> MEKIKVAIADDNKELVKTLESYLADHPQIEVITTAPNGKVILS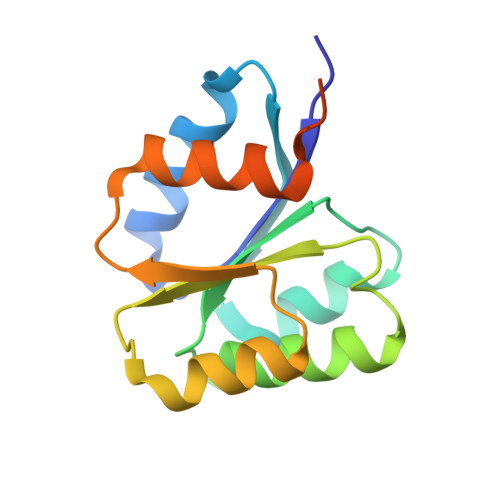LMENDLPDVLLLDIIMPHLDGLAVLEMMQANENLSKVQVIMLTAFGQEDVMKQAVDLGASYFMLKPFEFDRLVNQILQVAGHKQEADQRSSILQSQPQPKT One of the phosphatases responsible for plant phytochrome dephosphorylation and thereby increased activity is the phytochrome-associated protein phosphatase 5 (PAPP5). Studies by Ryu et al. have shown that the PP2A domain of PAPP5 dephosphorylates the NTE of AsPhyA and AtPhyB, whereas the TPR region binds to the C-terminal histidine kinase-related domain of AsPhyA. A C-terminal inhibitory motif blocks together with the TPR region the active site of the PP2A domain, where two catalytic manganese ions are bound. Like mammalian PP5, PAPP5 is activated by the polyunsaturated fatty acid arachidonic acid (AA).

We crystallized AtPAPP5 in a monoclinic crystal form that resulted in a dataset at 3.0 Å resolution. The AtPAPP5 structure shows the characteristic bilobal shape of a type 5 serine/threonine phosphatase with two manganese ions bound in the active site. Three TPR repeats (TPR1: V10-L42, TPR2: W50-V76 and TPR3: S81-L110) are linked via a long helical linker (P115-T173) to the PP2A domain (L174-N484). In contrast to mammalian PP5 structures in our AtPAPP5 structure the linker region is completely defined by electron density. Here, Mn2+ ion 1 is tetra-valently coordinated by amino acids D257, N289, H338 and H413, whereas Mn2+ ion 2 interacts with amino acids D228, H230 and D257. Instead, we observe a coordinated chloride ion in our AtPAPP5 structure. This partly occupied chloride (molecule A: 59%, B: 65%) replaces a phosphate anion that was observed before in the active site of the isolated PP2A domain of HsPP5. The AtPAPP5 structure represents the autoinhibited state, in which both the TPR region as well as the C-terminal inhibitory motif (K471-N484) block the active site and deny access for putative substrate-like phosphopeptides. Here, the prominent hydrogen bonds between the carboxylate group of E61 to Y437 and R261 are of particular interest, since both amino acids are involved in the coordination of the substrate’s phosphate group. The αJ-helix of the C-terminal inhibitory motif is indirectly involved in shielding the active site by stabilizing the closed-state interactions of the PP2A domain with the TPR region.

>[2x]MGSSHHHHHHSSLVPRGSHMMETKNENSDVSRAEEFKSQANEAFKGHKYSSAIDLYTKAIELNSNNAVYWANRAFAHTKLEEYGSAIQDASKAIEVDSRYSKGYYRRGAAYLAMGKFKDALKDFQQVKRLSPNDPDATRKLKECEKAVMKLKFEEAISVPVSERRSVAESIDFHTIEVEPQYSGARIEGEEVTLDFVKTMMEDFKNQKTLHKRYAYQIVLQTRQILLALPSLVDISVPHGKHITVCGDVHGQFYDLLNIFELNGLPSEENPYLFNGDFVDRGSFSVEIILTLFAFKCMCPSSIYLARGNHESKSMNKIYGFEGEVRSKLSEKFVDLFAEVFCYLPLAHVINGKVFVVHGGLFSVDGVKLSDIRAIDRFCEPPEEGLMCELLWSDPQPLPGRGPSKRGVGLSFGGDVTKRFLQDNNLDLLVRSHEVKDEGYEVEHDGKLITVFSAPNYCDQMGNKGAFIRFEAPDMKPNIVTFSAVPHPDVKPMAYANNFLRMFN> WS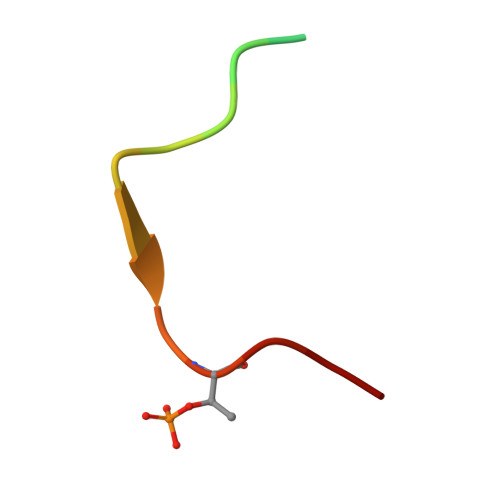SSLATPPTLSSTVLI>[4x]ARKCSLTGKWTNDLGSNMTIGAVNS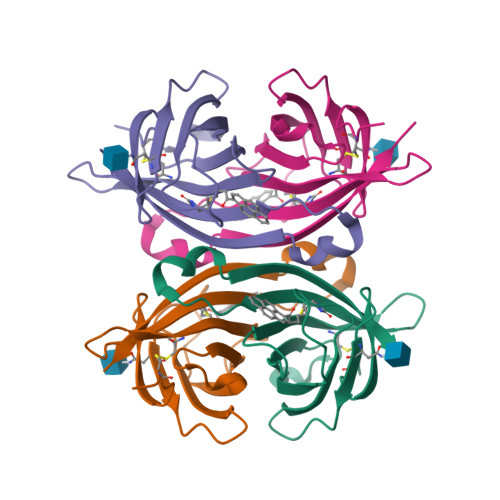RGEFTGTYTTAVTATSNEIKESPLHGTQNTINKRTQPTFGFTVNWKFSESTTVFTGQCFIDRNGKEVLKTMWLLRSSVNDIGDDWKATRVGINIFTRLRTQKE> VLFQGPPTKKVLDENGQSINGKSVLPNATLDYVAKQNFSQYKGIKASAEAIAKGFAFVDQPNEALAELTVKSIKASNGDDVSSLLEMRHVLSKDTLDQKLQSLIKEAGISPVGEFYMWTAKDPQAFYKAYVQKGLDITYNLSFKVKKEFTKGQIKNGVAQIDFGNGYTGNIVVNDLTTPEVHKDVLDKEDGKSINNDTVKLGDEVTYKLEGWVVPANRGYDLFEYKFVDHLQHTHDLYLKDKVVAKVAITLKDGTVIPKGTNLVQYTETVYNKETGRYELAFKADFLAQVSRSSAFGADDFIVVKRIKAGDVYNTADFFVNGNKVKTETVVTHTPEKPKPVMPQKVTPKAPALPSTGEQ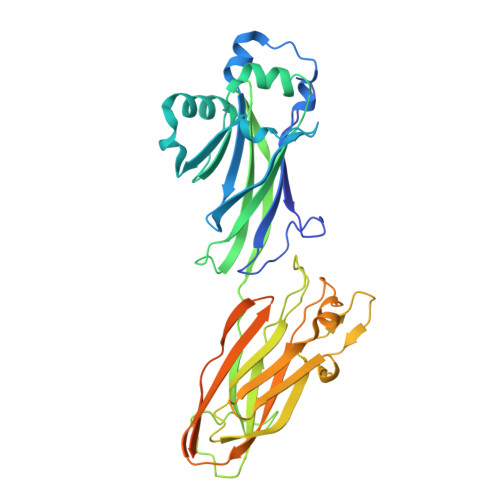GVSVLTVLGAALLSLLGLVGFKKRQQ> LRLLDHRALVCSQPGLNCTVKNSTCLDDSWIHPRNLTPSSPKDLQIQLHFAHTQQGDLFPVAHIEWTLQTDASILYLEGAELSVLQLNTNERLCVRFEFLSKLRHHHRRWRF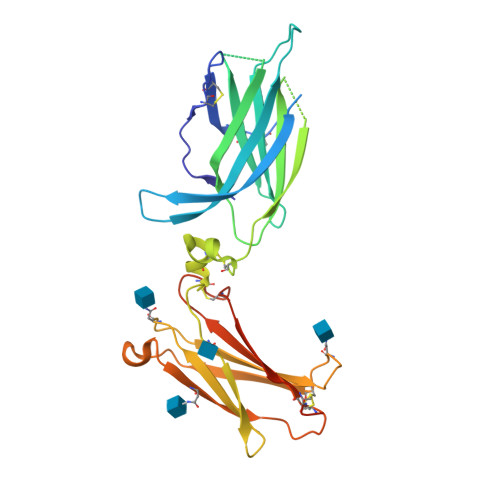TFSHFVVDPDQEYEVTVHHLPKPIPDGDPNHQSKNFLVPDCEHARMKVTTPCMSSGSLWDPNITVETLEAHQLRVSFTLWNESTHYQILLTSFPHMENHSCFEHMHHIPAPRPEEFHQRSNVTLTLRNLKGCCRHQVQIQPFFSSCLNDCLRHSATVSCPEMPDTPEPIPDYMP5-acetamido-2,6-anhydro-3,5-dideoxy-3-[(2E)-3-(4-methylphenyl)prop-2-en-1-yl]-D-glycero-D-galacto-non-2-enonic 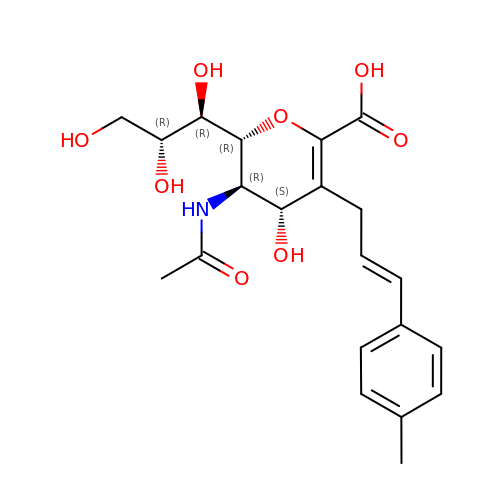acid | C21 H27 N O8 | CCPSTGRFUHTVNN-ZSEVYCOTSA-N>[2x]GMSSKAEKDIKWGIAPIGWRNDDIPSIGKDNNLQQLLSDIVVAGFQGTEV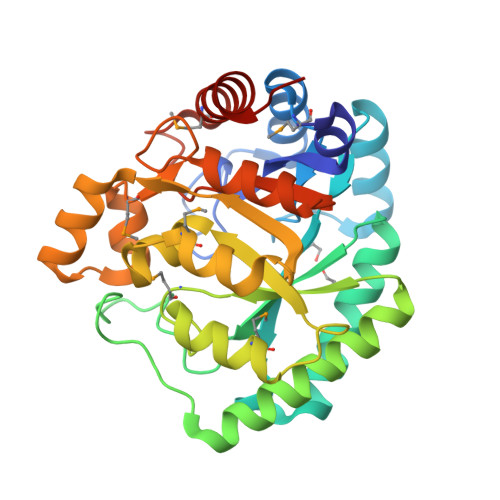GGFFPGPEKLNYELKLRNLEIAGQWFSSYIIRDGIEKASEAFEKHCQYLKAINAPVAVVSEQTYTIQRSDTANIFKDKPYFTDKEWDEVCKGLNHYGEIAAKYGLKVAYHHHMGTGIQTKEETDRLMANTDPKLVGLLYDTGHIAVSDGDYMALLNAHIDRVVHVHFKDVRRSKEEECRAKGLTFQGSFLNGMFTVPGDGDLDFKPVYDKLIANNYKGWIVVEAEQDPSKANPLEMAQIAHRYIKQHLIEN After transcription, the 3′-end is oligo-uridylylated by a terminal uridylyltransferase, TUT1 (TUTase6)910, one of the members of the non-canonical nucleotidyltransferases. TUT1 is composed of N-terminal Zn-finger, RRM, palm, fingers and KA-1 domains. The C-terminal region of TUT1 is a previously unidentified RNA-binding domain, and it was named the KA-1 domain. Thus, the present structural and biochemical studies have demonstrated that TUT1 acts as a U6 snRNA-specific terminal uridylyltransferase.

Therefore, the complex structures of TUT1_ΔN with either UTP or ATP soaked in were analysed. The structures of form-II TUT1_ΔN with UTP and ATP soaked in were also analysed, and the structures were modelled and refined to R factors of 22.9% (Rfree of 25.7%) and 24.1% (Rfree of 28.2%) for the UTP complex and the ATP complex, using reflections up to 2.7 and 2.8 Å resolutions, respectively. In the structure of UTP-bound TUT1_ΔN, one magnesium ion is coordinated by the β-γ phosphates of UTP and the catalytic Asp216 and Asp218 residues. The phosphate group of UTP forms hydrogen bonds with the Nη atom of Arg414, the Nδ atom of Asn432 and the main-chain amino-group of Asp216. The uracil base is sandwiched between Tyr432 and the side chain of Arg366. The O2 and O4 atoms of UTP form hydrogen bonds with the Nδ atom of Asn392 and the Nɛ atom of His549, respectively. The N3 atom of UTP forms a hydrogen bond with a water molecule that also hydrogen bonds with Asp543. The ribose 2′-OH of UTP forms hydrogen bonds with the Oδ atom of Asn392, thus discriminating the ribose from the deoxyribose. The structure of the TUT1 nucleotide-binding pocket is suitable for interactions with UTP, through specific hydrogen bonds between the uracil base and the conserved His and Asn residues in the catalytic pocket.

>[2x]MGAAPDSHQLAKALAEAADVGAQMIKLVGLRELSEAERQLRSLVVALMQEVFTEFFPGCVVHPFGSSINSFDVHGCDLDLFLDLGDLEEPQPVPKLPPASPLLEDREEGDLGKASELAETPKEEKAEGAAMLELVGSILRGCVPGVYRVQTVPSARRPVVKFAHRPSGLHGDVSLSNRLALHNSRFLSLASELDGRVRPLVYTLRAWAQGRGLSGSGPLLSNYALTLLVIYFLQTRDPPVLPTVSQLTQKAGEGEQVEVDGWDCSFPRDASRLEPSINVEPLSSLLAQFFSAVSSWDLRGSLLSLREGQALPVAGGLPSNLWEGLRLGPLNLQDPFDLSHNVAANVTSRVAGRLQNCCRAAANYARSLQYQRRSSRGRDWGLLPLLQPSSPSSLLSATPIPLPLAPFTQLTAALVQVFREALGCHIEQATKRTRSEGGGTGQGEAGKGASLPSSASWRCALWHRVWQGRRRARRRLQQQTKEGAGGGAGTRAGWLATEAQVTQELKGLSGGEERPETEPLLSFVASVSPADRMLTVTPLQDPQGLFPDLHHFLQVFLPQAIRHLKLEHHHHHH> AAMVLAYYSGYAGNYAALTRYAASFNAVAVDFYNITAQGAVTGNGDPAPNDAISFLLGRKIPAYGCVSNVDGNGNWSADIAHAVSTSAQSQAVANLVKFAQDKRFSGINVDFEAVAQGDRNNFSHFIQVLGRALHAKGLKLIVSVPAFSAKDENHPANYGYDLRALGAAADYLQIMSYDEAIPAWDPGPVAGSDWMEDDLDYAVERVPAAKILNGIPAYGYDWKRPGDGGMLYWKDTQALIARYGAQPRYDAGTHSLTFNYGAADGSRHTVWTENARSVALKASLVNAYGL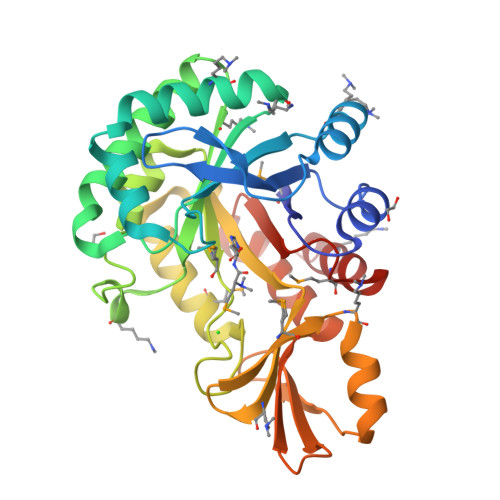GGTSLYALGMEDDAFWAAVKQGLAQR>[2x]SSPATSPQSTPTLVSALETIEPEVLYAGYDSSVPDSTWRIMTTLNMLGGRQVIAAVKWAKAIPGFRNLHLDDQMTLLQYSWMYLMAFALGWRSYRQSSANLLCFAPDLIINEQRMTLPDMYDQCKHMLYVSSELHRLQVSYEEYLCMKTLLLLSSVPKDGLKSQALFDAIRMTYIKELGKAIVKREGNSSQN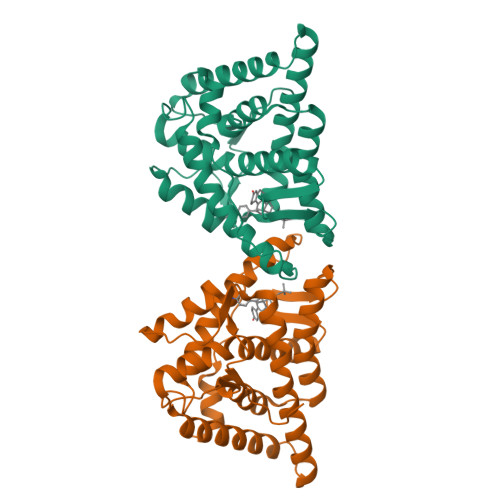SQRFYQLTKLLDSMHEVVENLLNYCFQTFLDKTMSIEFPEMLAEIITNQIPKYSNGNIKKLLFHQK1-[4-(piperazin-1-yl)pyridin-3-yl]-N-[(quinoxalin-6-yl)methyl]methanamine 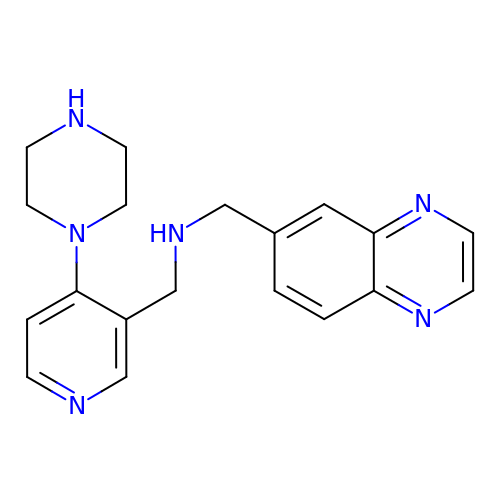| C19 H22 N6 | XFJFERUVHIMWDN-UHFFFAOYSA-N>MSGADRSPNAGAAPDSAPGQAAVASAYQRFEPRAYLRNNYAPPRGDLCNPNGVGPWKLRCLAQTFAT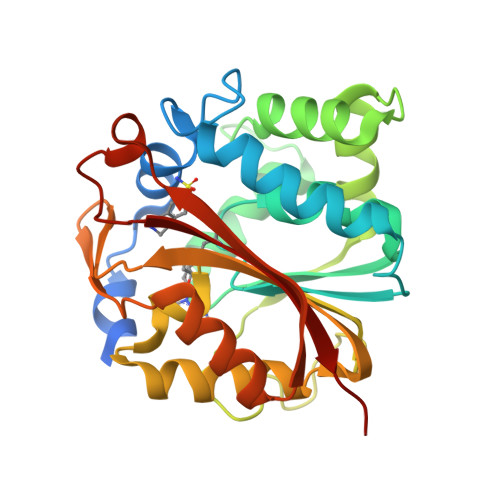GEVSGRTLIDIGSGPTVYQLLSACSHFEDITMTDFLEVNRQELGRWLQEEPGAFNWSMYSQHACLIEGKGECWQDKERQLRARVKRVLPIDVHQPQPLGAGSPAPLPADALVSAFCLEAVSPDLASFQRALDHITTLLRPGGHLLLIGALEESWYLAGEARLTVVPVSEEEVREALVRSGYKVRDLRTYIMPAHLQTGVDDVKGVFFAWAQKVGL[2x]Clostridium histolyticum collagenases ColG and ColH are segmental enzymes that are thought to be activated by Ca2+-triggered domain reorientation to cause extensive tissue destruction. The collagenases consist of a collagenase module (s1), a variable number of polycystic kidney disease-like (PKD-like) domains (s2a and s2b in ColH and s2 in ColG) and a variable number of collagen-binding domains (s3 in ColH and s3a and s3b in ColG). The X-ray crystal structures of Ca2+-bound holo s2a (space group C2), Ca2+-free apo s2a (space group P61), Ca2+-bound holo s2b (space group P21) and two new forms of N-terminally truncated wild-type apo s2 (space groups P21 and P212121) are reported for the first time. Comparison of crystal structures of ColG s2 with crystal structures of ColH s2a and s2b suggests that despite common tertiary folds, PKD-like domains can be grouped into two subsets.

Despite being solved in two crystal forms, the crystal structures of forms I and II of apo s2 from ColG are similar. Each asymmetric unit contains two noncrystallographic twofold symmetry-related molecules. All four molecules are virtually identical to each other (r.m.s.d. of <0.5 Å). Each structure begins at residue 685, although the first two residues (Gly-Ser) are remnants from GST-tag cleavage. The last residue is either 770 or 771. In apo s2, intermolecular antiparallel β-sheet interactions involving β-strand A could suppress dynamics of the region. Conversely, the PKD-like domain of collagenases consisting of multiple CBDs, such as s2, appears to have no surface aromatic residues. In contrast, the subset containing s2 is likely to be different; the lack of surface aromatic residues on s2 suggests that the domain is less directly involved in interactions with collagen. In this context, the spring-like dynamics of s2 may allow it to swell the fibril.

>[2x]GSAPIAKVTGPSTGAVGRNIEFSGKDSKDEDGKIVSYDWDFGDGATSRGKNSVHAYKKAGTYNVTLKVTDDKGATATESFTIEIKNE>GPHMARKFFVGGNWKCNGTAEEVKKIVNTLNE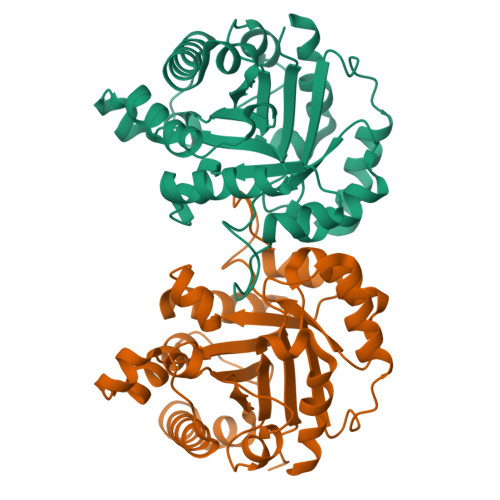AQVPSQDVVEVVVSPPYVFLPLVKSTLRSDFFVAAQNCWVKKGGAFTGEVSAEMLVNLDIPWVILGHSERRAILNESSEFVGDKVAYALAQGLKVIACVGETLEEREAGSTMDVVAAQTKAIADRVTNWSNVVIAYEPVWAIGTGKVASPAQAQEVHDELRKWLAKNVSADVAATTRIIYGGSVNGGNSKELGGQADVDGFLVGGASLKPEFIDIIKAAEVKKSA[4x]> MGSSHHHHHHSQDPNSMSQPFASRGLAWFQALAGSLAPRPGDPASLRVADAELDGYPVRFLAVVPDPDNPFPRARQGEVGLLEGWGLAAAVDEALEADREAPRKRALLAIVDVPSQAYGRREEALGIHQALAGAVDAYARARLAGHPLIGLLVGKAMSGAFLAHGYQANRLIALHDPGVMVHAMGKAAAARITLRSVEELEALAAKVPPMAYDIDSYASLGLLWRTLPVETVEVPSTADLVRVR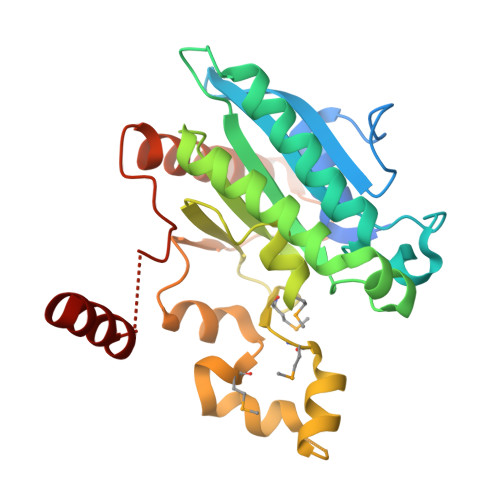TCLGEALADILGGPRDLGGRLGAANREASARVRRLLREQW> DLPRLIVYFQTTHDSSNRPISMLPLITEKGIALTHLIVCSFHINQGGVVHLNDFPPDDPHFYTLWNETITMKQAGVKVMGMVGGAAPGSFNTQTLDSPDSATFEHYYGQLRDAIVNFQLEGMDLDVEQPMSQQGIDRLIARLRADFGPDFLITLAPVASALEDSSNLSGFSYTALQQTQGNDIDWYNTQFYSGFGSMADTSDYDRIVANGFAPAKVVAGQLTTPEGAGWIPTSSLNNTIVSLVSEYGQIGGVMGWEYFNSLPGGTAEPWEWAQIVTVILRPGL

Endo-N-acetyl-β-D-glucosaminidases (ENGases, EC.3.2.1.96) hydrolyze the β-1,4 linkage in the chitobiose core of N-linked glycans and are thus capable of releasing entire glycans from glycoproteins leaving one N-acetylglucosamine residue on the substrate. The active site of the family 18 glycoside hydrolases contains two conserved acidic residues at the end of β-strand 4, corresponding to D129 and E131 in Endo T. The glutamic acid has been identified as the proton donor, and the aspartic acid has been assigned a secondary role, stabilizing the intermediate in a substrate-assisted hydrolysis mechanism in which the carbonyl oxygen group of the C2-acetamido of the leaving N-acetyl-D-glucosamine (GlcNAc) acts as the nucleophile. In this study, the 1.3 Å crystal structure is described as the first fungal representative in GH family 18 with endo-N-acetyl-β-D-glucosaminidase activity, Endo T from H. jecorina. The mannosyl glycoprotein endo-N-acetyl-β-D-glucosaminidase (Endo T, HjEng18A) is shown to be responsible for the microheterogeneity observed for Hypocrea jecorina cellulases and hemicellulases.

The final Endo T structure model, based on the 1.3 Å high resolution native dataset, contains 2237 non-hydrogen atoms belonging to one protein molecule consisting of 283 amino acid residues, two N-acetylglucosamine residues, seven zinc ions and 434 water molecules and 3 acetate molecules. Although 46 amino acids are missing at the C-terminus of the protein, the overall fold of Endo T is a complete (β/α)8-TIM barrel. Seven zinc atoms have been modeled in the structure model of Endo T, six of which are located at the surface of the molecule. The seventh zinc atom is bound deep in the active site of the enzyme in a pocket formed by the catalytic residues. This zinc atom has dual conformations in the structure model and it is coordinated by the two catalytic residues. The Endo T structure also shows two single GlcNAc residues bound at two of the predicted N-glycosylation sites of the enzyme, N70 and N240 respectively. In Endo T, the conserved tyrosine Y195 is present in an almost identical position and a zinc atom is found bound at the exact same position where the reducing GlcNAc molecule is found in the Endo F3 structure. The β3α3 loop is relatively long in all compared structures and is located next to the catalytic acids. This loop shows a lot of structural variation among the five structures: Endo F3 has an α-turn in this loop, Endo H, Endo F1 and Endo BT have a much shorter loop, while in Endo T this loop is highly structured and actively takes part in building up the active site of the enzyme. The overall comparison of the five structures shows that Endo T possesses a slightly deeper and narrower substrate-binding cleft than the other enzymes.> ETGKPTCDEKYANITVDYLYNKETKLFTAKLNVNENVECGNNTCTNNEVHNLTECKNASVSISHNSCTAPDKTLILDVPPGVEKFQLHDCTQVEKADTTICLKWKNIETFTCDTQNITYRFQCGNMIFDNKEIKLENLEPEHEYKCDS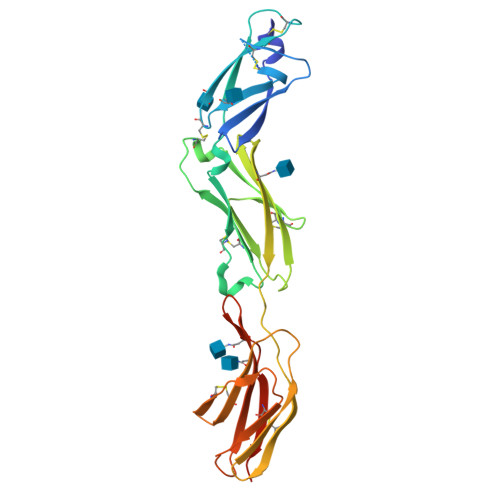EILYNNHKFTNASKIIKTDFGSPGEPQIIFCRSEAAHQGVITWNPPQRSFHNFTLCYIKETEKDCLNLDKNLIKYDLQNLKPYTKYVLSLHAYIIAKVQRNGSAAMCHFTTKGTKHHHHHH>[4x]GMNGMLLSRIKKKAMELAEDLKLVDFSFGLPYTWVLVEGIEGRALGVAMTLPEEVQRYTNSIEEPSLLEFIDKADSLNIIERTLGVAAINAVSQYYIDLREAKWIDVTEL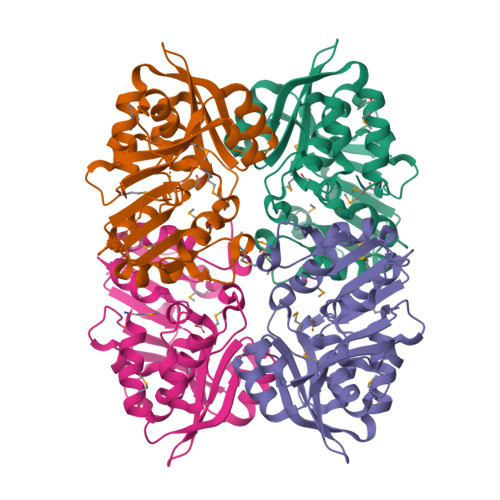IQQDEIKRIAIIGNMPPVVRTLKEKYEVYVFERNMKLWDRDTYSDTLEYHILPEVDGIIASASCIVNGTLDMILDRAKKAKLIVITGPTGQLLPEFLKGTKVTHLASMKVTNIEKALVKLKLGSFKGFESESIKYVIEV> VQFGVMIEKMTGKSALQYNDYGCYCGIGGSHWPVDQ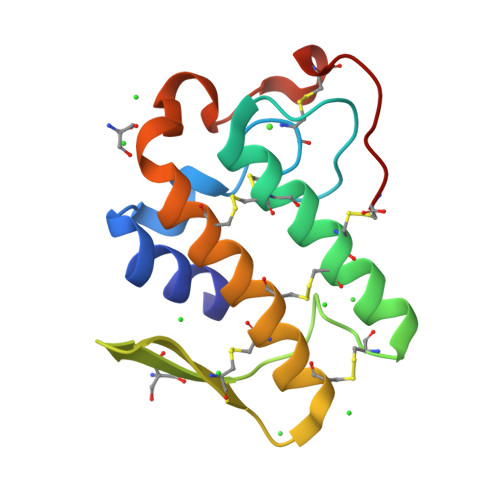TDWCCHAHDCCYGRLEKLGCEPKLEKYLFSVSERGIFCAGRTTCQRLTCECDKRAALCFRRNLGTYNRKYAHYPNKLCTGPTPPC> LPVLAPVTKDPATSLYTIPFHDGASLVLDVAGPLVWSTCDGGQPPAEIPCSSPTCLLANAYPAPGCPAPSCGSDKHDKPCTAYPYNPVSGACAAGSLSHTRFVANTTDGSKPVSKVNVGVLAACAPSKLLASLPRGSTGVAGLANSGLALPAQVASAQKVANRFLLCLPTGGPGVAIFGGGPVPWPQFTQSMPYTPLVTKGGSPAHYISARSIVVGDTRVPVPEGALATGGVMLSTRLPYVLLRPDVYRPLMDAFTKALAAQHANGAPVARAVEAVAPFGVCYDTKTLGNNLGGYAVPNVQLGLDGGSDWTMTGKNSMVDVKQGTACVAFVEMKGVAAGDGRAPAVILGGAQMEDFVL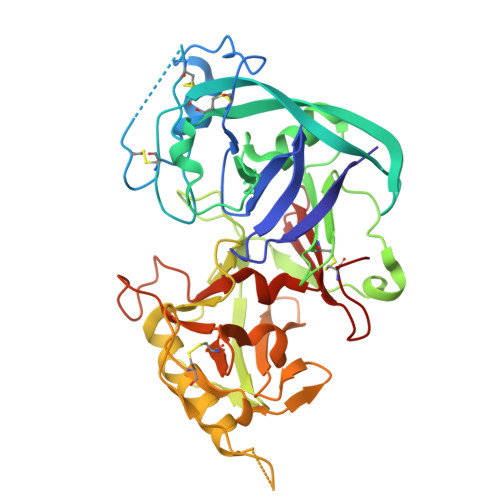DFDMEKKRLGFSRLPHFTGCGGL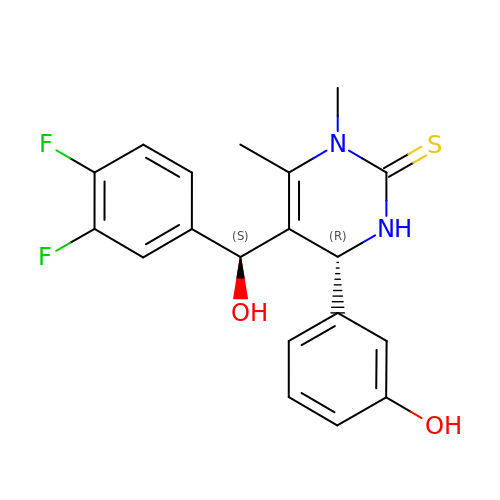(4R)-5-[(S)-(3,4-DIFLUOROPHENYL)(HYDROXY)METHYL]-4-(3-HYDROXYPHENYL)-1,6-DIMETHYL-3,4-DIHYDROPYRIMIDINE-2(1H)-THIONE | C19 H18 F2 N2 O2 S | WGZRWWKQRQTPSR-MSOLQXFVSA-N> PGPVPPSTALRELIEELVNITQNQKAPLCNGSMVWSINLTTAGMYCAALESLINVSGCSAIEKT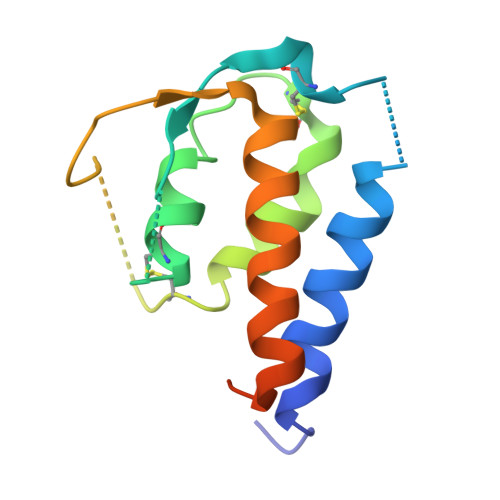QRMLSGFCPHKVSAGQFSSLHVRDTKIEVAQFVKDLLLHLKKLFREGQFNRNFESIIICRDRT> MKRIPRKTKGKSSGKGNDSTERSDDGSSQLRDKQNNKAGPATTEPGTSNREQYRARPGIASVQRATESAELPMKNNDEGTPDKKGNTRGDLVNEHSEAKDEADEATQKQAKDTDKSKAQVTYSDTGINNANELSRSGNVDNEGGSNQKPMSTRIAEATSAIVSKHPARVGLPPTASSGHGYQCHVCSAVLFSPLDLDAHVASHGLHGNMTLTSSEIQRHITEFISSWQNHPIVQVSADVENKKTAQLLHADTPRLVTWDAGLCTSFKIVPIVPAQVPQDVLAYTFFTSSYAIQSPFPEAAVSRIVVHTRWASNVDFDRDSSVIMAPPTENNIHLFKQLLNTETLSVRGANPLMFRANVLHMLLEFVLDNLYLNRHTGFSQDHTPFTEGANLRSLPGPDAEKWYSIMYPTRMGTPNVSKICNFVASCVRNRVGRFDRAQMMNGAMSEWVDVFETSDALTVSIRGRWMARLARMNINPTEIEWALTECAQGYVTVTSPYAPSVNRLMPYRISNAERQISQIIRIMNIGNNATVIQPVLQDISVLLQRISPLQIDPTIISNTMSTVSESTTQTLSPASSILGKLRPSNSDFSSFRVALAGWLYNGVVTTVIDDSSYPKDGGSVTSLENLWDFFILALALPLTTDPCAPVKAFMTLANMMVGFETIPMDNQIYTQSRRASAFSTPHTWPRCFMNIQLISPIDAPILRQWAEIIHRYWPNPSQIRYGAPNVFGSANLFTPPEVLL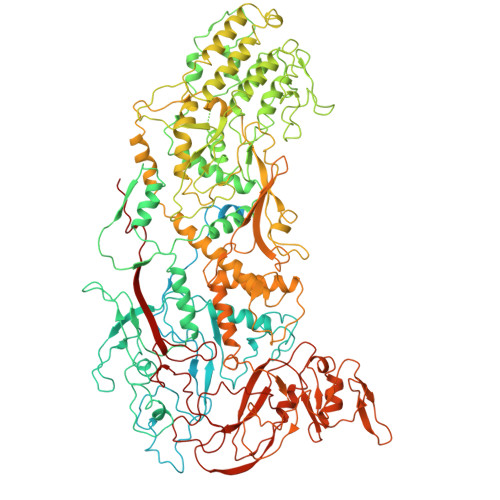LPIDHQPANVTTPTLDFTNELTNWRARVCELMKNLVDNQRYQPGWTQSLVSSMRGTLDKLKLIKSMTPMYLQQLAPVELAVIAPMLPFPPFQVPYVRLDRDRVPTMVGVTRQSRDTITQPALSLSTTNTTVGVPLALDARAITVALLSGKYPPDLVTNVWYADAIYPMYADTEVFSNLQRDMITCEAVQTLVTLVAQISETQYPVDRYLDWIPSLRASAATAATFAEWVNTSMKTAFDLSDMLLEPLLSGDPRMTQLAIQYQQYNGRTFNVIPEMPGSVIADCVQLTAEVFNHEYNLFGIARGDIIIGRVQSTHLWSPLAPPPDLVFDRDTPGVHIFGRDCRISFGMNGAAPMIRDETGMMVPFEGNWIFPLALWQMNTRYFNQQFDAWIKTGELRIRIEMGAYPYMLHYYDPRQYANAWNLTSAWLEEITPTSIPSVPFMVPISSDHDISSAPAVQYIISTEYNDRSLFCTNSSSPQTIAGPDKHIPVERYNILTNPDAPPTQIQLPEVVDLYNVVTRYAYETPPITAVVMGVP>[2x]QSMSKSAVSPMMQQYLGIKAQHTDKLVFYRMGDFYELFLDDAVEAAKLLDITLTTRGQMDGVPIKMAGVPFHAAEQYLARLVKLGKSVAICEQVGEVGAGKGPVERKVVRIVT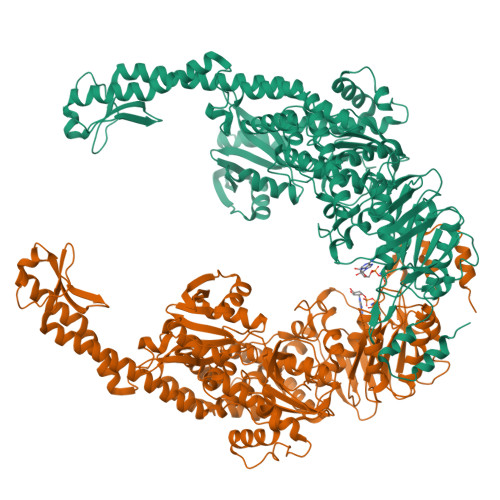PGTLTDSALLEDKETNRIVAVSPDKKYIGLAWASLQSGEFKTKLTTADKLNDELARLQAAEILLPDSKNAPQLQTASGVTRLNAWQFAADAGEKLLTEYFGCQDLRGFGLDSKEHAVSIGAAGALLNYIRLTQNLMPQHLDGLSLETDSQYIGMDAATRRNLEITQTLSGKKTPTLFSILDGCATHMGSRLLALWLHHPLRNRAHIRARQEAVTALESQYEPLQCHLKSIADIERIAARIAVGNARPRDLASLRDSLFELAQIDLSATGSSLLETLKAVFPETLPVAETLKAAVMPEPSVWLKDGNVINHGFHPELDELRRIQNHGDEFLLDLEAKERERTGLSTLKVEFNRVHGFYIELSKTQAEQAPADYQRRQTLKNAERFITPELKAFEDKVLTAQDQALALEKQLFDGVLKNLRTALPQLQKAAKAAAALDVLSTFSALAKERNFVRPEFADYPVVHIENGRHPVVEQQVRHFTANHTDLDHKHRLMLLTGPNMGGKSTYMRQVALIVLLAHTGCFVPADAATIGPVDQIFTRIGASDDLASNRSTFMVEMSETAYILHHATEQSIVLMDEVGRGTSTFDGLALAHAIAEHLLQKNKSFSLFATHYFELTYLPEAHAAAVNMHLSALEQGRDIVFLHQIQPGPAGKSYGIAVAKLAGLPVRALKAAQKHLNGLENQAAANRPQLDIFSTMPSEKGDEP>HHHHHHMEKKLSDAQVALVAAWRKYPDLRESLEEAASILSLIVFQAETLSDQANELANYIRRQGLEEAEGACRNIDIMRAKWVEVCGEVNQYGIRVYGDAIDRDVD[4x]

One mechanism by which phages and other mobile genetic elements are able to overcome the CRISPR-Cas system is through the expression of anti-CRISPR proteins. We previously reported that gene 34 from Pseudomonas phage JBD5, which encodes the protein AcrE1, shows anti-CRISPR activity against the type I-E system of P. aeruginosa strain SMC4386 (4). We show that AcrE1 binds to the CRISPR-associated helicase/nuclease Cas3 and that the C-terminal region of the anti-CRISPR protein is important for its inhibitory activity. In summary, these experiments demonstrate that AcrE1 functions by blocking the activity of Cas3 without inhibiting the DNA-binding activity of Cascade.

(c) Structural overlay of the X-ray crystal structures of the AcrE1 proteins with an N-terminal (blue) and C-terminal (red) 6×His tag reveals virtually identical structures. Thus, the unusual nature of the C-terminal sheet was not a result of the presence of the 6×His affinity purification tag fused to the C terminus. The C-terminal β-sheet region is unusual because both sides of the sheet are exposed to solvent, contrasting with typical β-sheets, which pack a hydrophobic surface on one side against helices or other sheets. We also examined the packing of the C-terminal β-sheet within the crystal and observed no contacts that stabilize it in this position. Residues 82 to 90 form an antiparallel β-sheet that protrudes at a 90° angle from the end of helix 3. This sheet structure appears to be stabilized by multiple interactions between residues at the base of the sheet and residues in helices 1, 2, and 3. A salt bridge is formed between E41 and R89.> MPIKGTSGSNIARPRFYNTVMVETIEGANAEERYFNPGELSSMAGFFNDAQRRLAIVQILTTNAEAIVSRAAGRIFTGGSPMAFSVQQANRQKDAEKERVSARVVQAESEQPIGNEVVIEDKGGFLERLKSFFSYGGAEVETPGFRPIPIAVYGPERMQKSLRDLDWFLRYVNYSLVAGDSNMILLNCLGLREILEKACSIDATIVAVQEMRRAATGYLKSNDDKELVGSYFDVIIRSLNADKSDTPADVVRPSSPDRAGLVLPAIYALAGQSRPAFKMSRTLTSAEKERVVRAAYRQVFERDILAYGQSISYLDSKVKNGEISVKEFIRLLGKSELYRKQFFEPFINSRVLELAFKHFLGRAPESRTEVQNYYSIVAAQGLGGLVDALVDGEEYGRIFGEDTVPFIRDLGQEAQPSWNWGAAYSLYNYAAPRRKVPQFITLYADYVKPLPNQHPYGSGNDPLEIQFGAIFKSETKAPSARPAPIGKDVQRILIRSGNPITNERGNPAGGISDKTSLSPQIFKLTQDNRRIRGKSGKGSLITNAGAGSVEVNVQAVIRAAYQQVFGRQLYEGQHLSVSEIKLENGEISVKEFVRDLATSEIFRKLYWQNFYVCKSIEYIHRRLLGRPTYGRDETNRYYDLAFKKGFAGVVNAILDTMEYAEVFGDDVVPYERYVTPAGLNLRKLRAGTVPTLPSFEETPKFIEKGTAPDRALPQIRSAINQGVSKKRDQRKIFSTVGIQTSLASRTEFDALIRAAYRQVFERDMDSYRITEVFSVLETKLRNREITTKEFIQALASSDLYRKQFFEPYPPTKNVELSLKHLLGRATKDQAELRKYNQIIATQGFKPFINAILDSKEYGEVFGDGTVPYNRYPTLPAANFPNTEILYNQLTKQSAEVVVPSFKPVTSPRGMDMSQTPLMLQAMGDIAEAEQEVALQKPLFIQKGKALRGAEGDPYTIGTRRSPKPIFWVPQGGTNPTEFQNVIRAAYRQVFERDVPDYQRLSYPESRLKNGEISMREFIRQLAESDLYRKQFYEPYPNTKVIELLTKHFLGRAPQDQAEIQRYNRILAGKGLKVAIEEVLNSDEYTQLFGEDVVPFKRYPTLPTGTYLASVATNDEMIQQSGSSYSPSYAGYSYPFS;>MSVVTKAIVSADAEARYLSPGELDRIRGFVSSGERRLRVAQTLTESRERIIKQAGDQLFQKRPDLVSPGGNAYGAERTASCLRDLDYYLRLVTFGIVAGDVTPIEEIGVIGVKEMYRNLEVPLPGMVEAVKAMKSVATGLLSGDDSAEVGYYFDYLAGALA[23x];> MQDVIGKVIAEYDTKGKYLDAAALDLLRSYFDSGDLRLKAAQAITANAEVIVRAASAKALHYTPVTKPGGNMYYARRYASCIRDLDYFLRYATYAMLADNTTLLDEYVLKGLTETYRALGVPLDISVRAINALKEVVAGQVGPKAGQEMAKYFDHLAKGLG;>[23x]MQDAITSVINTYDVQGKYFDTSAFDKLKAYYATGELRVRAAGTISANAATIIKEASAKLFSNQPDLVRPGGNAYTTRRYAACVRDMDYFLRYATYAMLAGDTSILDERVLNGLKETYNSLGVPISSTVQGIQAMKEVTGSLVGSGAAKEMGVYFDYLSSGLS;>MTRLFKVTALIPSYKKVRGGRELQNTYFTKLVEYDRWFAEQQRIQKQGGKILSVKMVAGKPGLNTGVL[4x]

Phycobilisomes (PBS) are antenna megacomplexes that transfer energy to photosystems II and I in thylakoids. Here we show the cryo-EM structure at a global resolution of 2.9 Å of the 5.9-MDa PBS from Anthocerotibacter panamensis (hereafter A. panamensis), a recently discovered Gloeobacterial species that diverged from Gloeobacter spp. around 1.4 billion years ago. The A. panamensis PBS features a configuration comprising two herein characterized linkers and presents a paddle-shaped morphology. The two-fold symmetric PBS contains twelve APC hexamers assembled as a heptacylindrical core surrounded by twelve PC hexamers, with approximate dimensions of 273 Å (width), 500 Å (height), and 129 Å (thickness).

The heptacylindrical core in A. panamensis has two distinct complexes—the bottom pentacylindrical and the top bicylindrical subcomplexes—each with a different combination of Apc protein components. Instead, ApcA2, ApcB2, ApcB3, ApcC2, and ApcE form the bottom pentacylindrical core, and these five proteins are phylogenetically close to their homologs in crown Cyanobacteria. However, both ApcD and ApcF are absent in the A. panamensis PBS. Although ApcB3 only exists as a single copy like ApcF of hemidiscoidal PBS in each bottom core cylinder, ApcB2 (β3) is found at the positions occupied by ApcF in other pentacylindrical core structures and is likely the functional equivalent to ApcF that occurs in crown Cyanobacteria. Additionally, the position of ApcD is occupied by an ApcA2 (α1) subunit in the paddle-shaped PBS. The linker proteins were suggested to provide microenvironments for the bilins and are key bridges in energy transfer in PBS, namely the linker-guided pathway. Both linker-guided and non-linker-guided pathways are identified in the pentacylindrical core. The final overall resolution of APC core complexes ranged from 2.38 Å to 2.73 Å, allowing the assignment of all APC subunits precisely based on the corresponding amino acid sequences.> GPGFDFAQAIMKKNTVVARTEKGEFTMLGVHDRVAVIPTHASVGETIYINDVETKVLDACALRDLTDTNLEI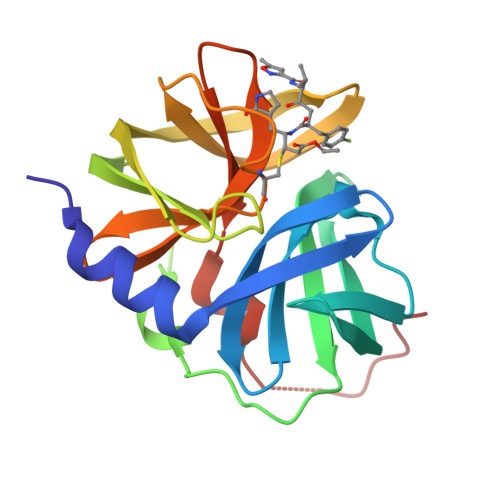TIVKLDRNQKFRDIRHFLPRYEDDYNDAVLSVHTSKFPNMYIPVGQVTNYGFLNLGGTPTHRILMYNFPTRAGQCGGVVTTTGKVIGIHVGGNGAQGFAAMLLHSYFTDTQKHHHHHH>[2x]TAVVQRVEIHKLRQGENLILGFSIGGGIDQDPSQNPFSEDKTDKGIYVTR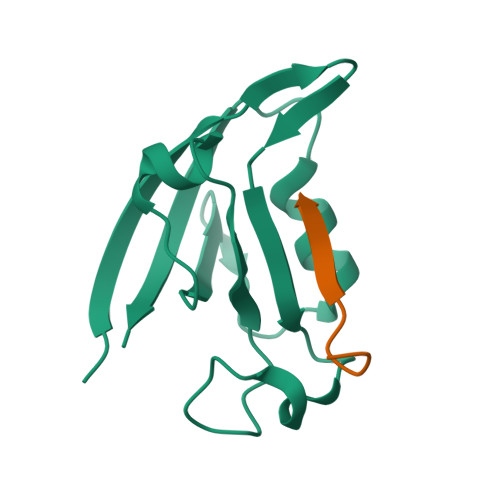VSEGGPAEIAGLQIGDKIMQVNGWDMTMVTHDQARKRLTKRSEEVVRLLVTRQ;>ANSRFPTSII[2x]>[2x]MGSSHHHHHHSSGLVPRGSSSTDFGDLVLLIGDLKIPYGAKELPSNFRELLATDKINYVLCTGNVCSQEYVEMLKNITKNVYIVSGDLDSAIFNPD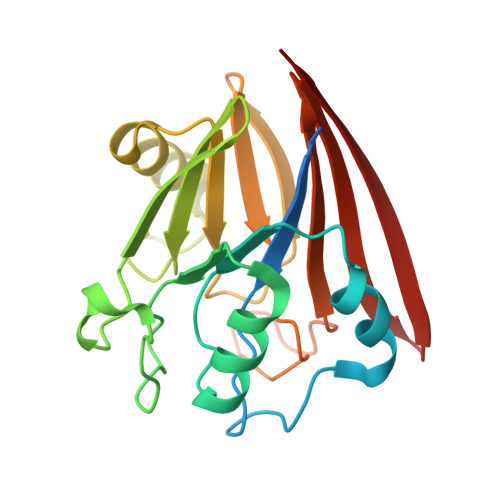PESNGVFPEYVVVQIGEFKIGLMHGNQVLPWDDPGSLEQWQRRLDCDILVTGHTHKLRVFEKNGKLFLNPGTATGAFSALTPDAPPSFMLMALQGNKVVLYVYDLRDGKTNVAMSEFSK>MAHHHHHHMTSTATSSPRVITSSPVVVALDYDNRDKALAFVERIDPRDCRLKVGKEMFTLLGPQFVR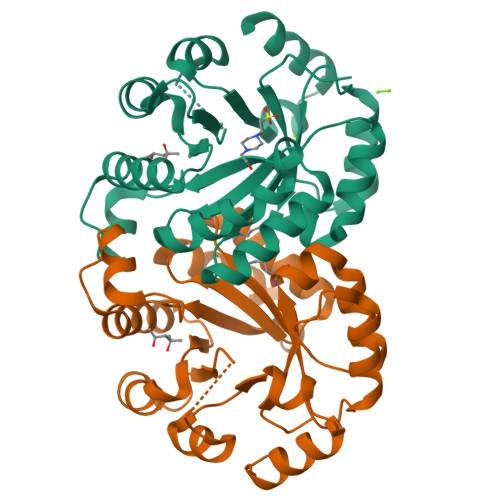DLHQRGFEVFLDLKFHDIPNTTARAVAAAAELGVWMVNVHASGGARMMTAAREALLPFGKEAPLLIAVTVLTSMEASDLQDLGIMLSPADHAAKLAALTKRCGLDGVVCSAQEAVRFKQELGQEFKLVTPGIRPTGSDAGDQRRIMTPEQAQQAGVDYMVIGRPVTQSADPVATLASINASLNKGV[6x]>GNTVTIDFMSADGIVPGRTPVRYQGVEVGTVQDISLSDDLRKIEVKVSIKSDMKDALREETQFWLVTPKASLAGVSGLDALVGGNYIGMMPGKGKEQDHFVALDTQPKYRLDNGDLMIHLQAPDLGSLNSGSLVYFRKIPVGKVYDYAINPNKQGVVIDVLIERRFTDLVKKGSRFWNVSGVDANVSISGAKVKLESLAALVNGAIAFDSPEESKPAEAEDTFGLYEDLAHSQRGVIIKLELPSGAGLTADSTPLMYQGLEVGQLTKLDLNPGGKVTGEMTVDPSVVTLLRENTRIELRNPKLSLSDANLSALLTGKTFELVPGDGEPRKEFVVVPGEKALLHEPDVLTLTLTAPESYGIDAGQPLILHGVQVGQVIDRKLTSKGV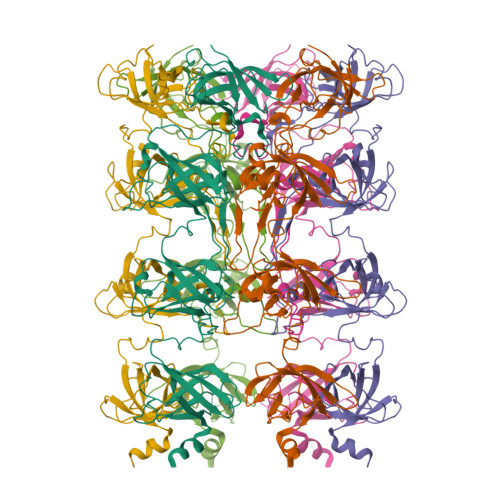TFTVAIEPQHRELVKGDSKFVVNSRVDVKVGLDGVEFLGASASEWINGGIRILPGDKGEMKASYPLYANLEKALENSL[6x]>[4x]GSSHHHHHHSSGENLYFQGHMTCPFADPAALYSRQDTTSGQSPLAAYEVDDSTGYLTSDVGGPIQDQTSLKAGIRGPTLLEDFMFRQKIQHFDHERVPERAVHARGAGAHGTFTSYADWSNITAASFLNATGKQTPVFVRFSTVAGSRGSADTARDVHGFATRFYTDEGNFDIVGNNIPVF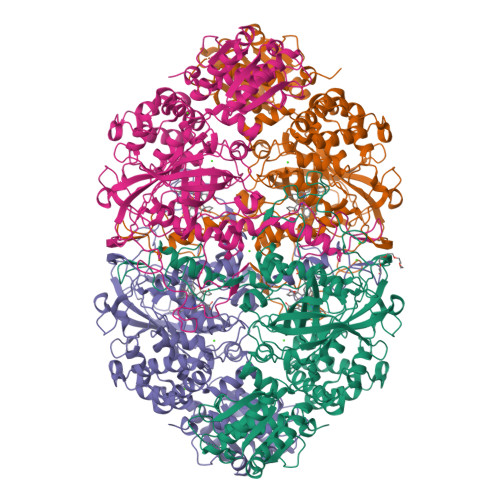FIQDAIQFPDLIHSVKPRPDNEIPQAATAHDSAWDFFSQQPSTMHTLFWAMSGHGIPRSYRHMDGFGVHTFRFVKDDGSSKLIKWHFKSRQGKASLVWEEAQVLSGKNADFHRQDLWDAIESGNGPEWDVCVQIVDESQAQAFGFDLLDPTKIIPEEYAPLTKLGLLKLDRNPTNYFAETEQVMFQPGHIVRGIDFTEDPLLQGRLFSYLDTQLNRNGGPNFEQLPINMPRVPIHNNNRDGAGQMFIHRNKYPYTPNTLNSGYPRQANQNAGRGFFTAPGRTASGALVREVSPTFNDHWSQPRLFFNSLTPVEQQFLVNAMRFEISLVKSEEVKKNVLTQLNRVSHDVAVRVAAAIGLGAPDADDTYYHNNKTAGVSIVGSGPLPTIKTLRVGILATTSESSALDQAAQLRTRLEKDGLVVTVVAETLREGVDQTYSTADATGFDGVVVVDGAAALFASTASSPLFPTGRPLQIFVDAYRWGKPVGVCGGKSSEVLDAADVPEDGDGVYSEESVDMFVEEFEKGLATFRFTDRFALDS>ATPADWRSQSIYFLLTDRFARTDGSTTATCNTADQKYCGGTWQGIIDKLDYIQGMGFTAIWITPVTAQLPQTTAYGDAYHGYWQQDIYSLNENYGTADDLKALSSALHERGMYLMVDVVANHMGYDGAGSSVDYSVFKPFSSQDYFHPFCFIQNYEDQTQVEDCWLGDNTVSLPDLDTTKDVVKNEWYDWVGSLVSNYSIDGLRIDTVKHVQKDFWPGYNKAAGVYCIGEVLDGDPAYTCPYQNVMDGVLNYPIYYPLLNAFKSTSGSMDDLYNMINTVKSDCPDSTLLGTFVENHDNP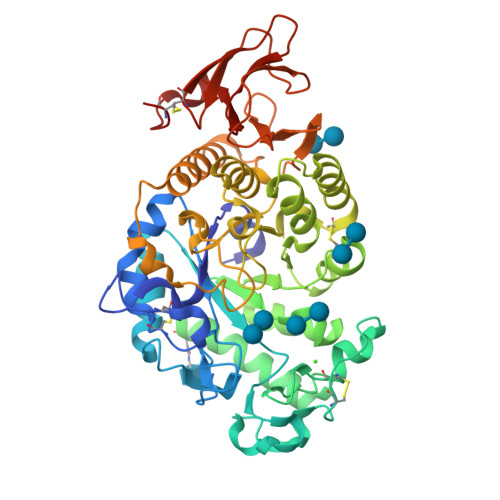RFASYTNDIALAKNVAAFIILNDGIPIIYAGQEQHYAGGNDPANREATWLSGYPTDSELYKLIASANAIRNYAISKDTGFVTYKNWPIYKDDTTIAMRKGTDGSQIVTILSNKGASGDSYTLSLSGAGYTAGQQLTEVIGCTTVTVGSDGNVPVPMAGGLPRVLYPTEKLAGSKICSSS[2x]>GH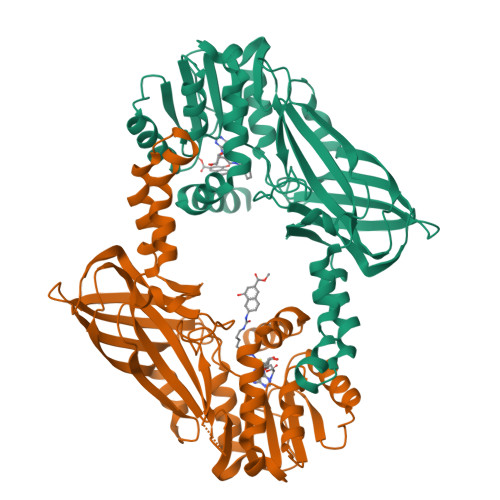MAAPPRPRRTKSERDQLYYESYSDVSVHEEMIADQVRTEAYRLGILKNWAALRGKTVLDVGAGTGILSIFCAQAGARRVYAVEASAIWQQAREVVRLNGLEDRVHVLPGPVETVELPERVDAIVSEWMGYGLLHESMLSSVLHARTKWLKEGGLLLPASAELFVAPISDQMLEWRLGFWSQVKQHYGVDMSCMESFATRCLMGHSEIVVQDLSGEDVLARPQRFAQLELARAGLEQELEAGVGGRFRCSCYGSAPLHGFAVWFQVTFPGGDSEKPLVLSTSPLHPATHWKQALLYLNEPVPVEQDTDISGEITLLPSPDNPRRLRILLRYKVGDHEEKTKDFAMED[2x]>MTSVTSKQSTILGSDEIDLGRVIGELIDHRKLIISITSVFTLFAILYALLATPIYETDALIQIEQKQGNAILSSLSQVLPDGQPQSAPETALLQSRMILGKTIDDLNLQIQIEQKYFPVIGRGLARLMGEKPGNIDITRLYLPDSDDISNNTPSIILTVKDKENYSINSDGIQLNGVVGTLLNEKGISLLVNEIDAKPGDQFVITQLPRLKAISDLLKSFSVADLGKDTGMLTLTLTGDNPKRISHILDSISQNYLAQNIARQAAQDAKSLEFLNQQLPKVRAELDSAEDKLNAYRKQKDSVDLNMEAKSVLDQIVNVDNQLNELTFREAEVSQLYTKEHPTYKALMEKRQTLQEEKSKLNKRVSSMPSTQQEVLRLSRDVESGRAVYLQLLNRQQELNIAKSSAIGNVRIIDNAVTDPNPVRPKKTIIIVIGVVLGLIVSVVLVLFQVFLRRGIESPEQLEEIGINVYASIPISEWLTKNARQSGKVRKNQSDTLLAVGNPADLAVEAIRGLRTSLHFAMMEAKNNVLMISGASPSAGMTFISSNLAATIAITGKKVLFIDADLRKGYAHKMFGHKNDKGLSEFLSGQAAAEMIIDKVEGGGFDYIGRGQIPPNPAELLMHPRFEQLLNWASQNYDLIIIDTPPILAVTDAAIIGRYAGTCLLVARFEKNTVKEIDVSMKRFEQSGVVVKGCILNGVVKKASSYYRYGHNHYGESEEDKKHHHHHH[8x]

Wzc, an integral cytoplasmic membrane tyrosine autokinase protein serves as the master regulator of the biosynthesis and export of many bacterial capsular polysaccharides and exopolysaccharides. Wzc comprises a large periplasmic domain, two transmembrane helices and a C-terminal cytoplasmic kinase domain with a tyrosine-rich tail. Wzc regulates polymerisation functions through cycling the formation and dissociation of an octameric complex, driven by changes in the phosphorylation status of the tyrosine-rich tail. E. coli Wzc serves a model for a wider family of polysaccharide co-polymerases.

Here, we report the characterisation of the structures WzcK540M2YE (Y718E, Y717E), WzcK540M3YE (Y718E, Y717E and Y715E) and WzcK540M3YE_N711Y (an additional N711Y mutation) corresponding to different phosphorylation states. One intermediate, 2pY which has Y713 at the active site, does not follow the YxY pattern, since position 711 is asparagine. Notably in the WzcK540M3YE structure the stretch of residues connecting the α23 to the active site is entirely disordered and molecular dynamics of 2pY showed this stretch of residues to be highly mobile. We show that it is binding of the i-2 tyrosine to the tyrosine pocket (where i is the number of the residue positioned at the kinase active site) orders the tail between the tyrosine at the active site and helix α23. The structural and MD data reported here confirm this hypothesis, showing that the tyrosine most stably positioned at the active site is the one immediately N-terminal to the phosphotyrosine (or the engineered Tyr-to-Glu mutation).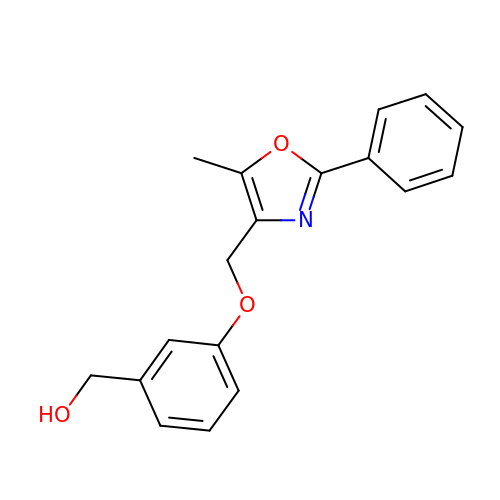{3-[(5-methyl-2-phenyl-1,3-oxazol-4-yl)methoxy]phenyl}methanol | C18 H17 N O3 | UPVJJOGZAKVERR-UHFFFAOYSA-N(2~{R})-2-methyl-2-[[2-methyl-3-oxidanyl-5-(phosphonooxymethyl)pyridin-4-yl]methylamino]-3-oxidanyl-propanoic acid | C12 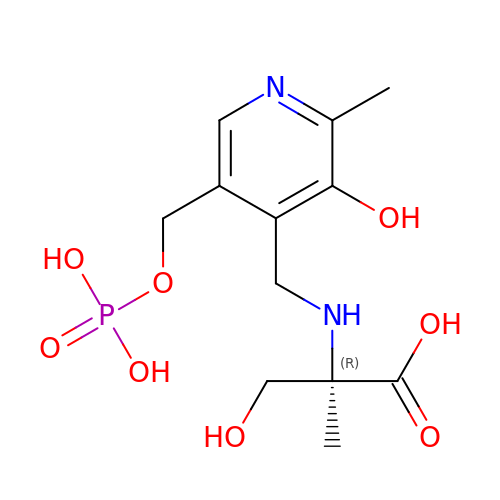H19 N2 O8 P | FVZJSLHHGJVQIU-GFCCVEGCSA-N> MGSSHHHHHHSQDPMLNSFKLSLQYILPKLWLTRLAGWGASKRAGWLTKLVIDLF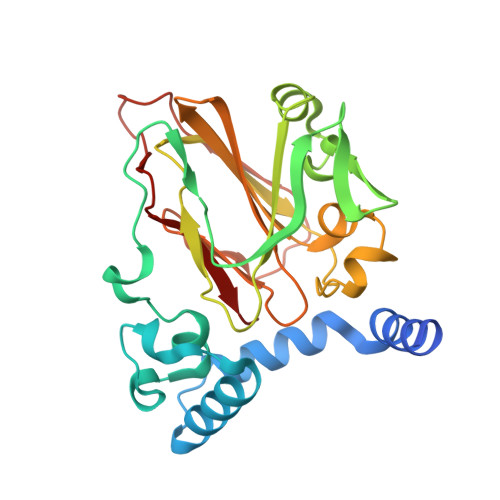VKYYKVDMKEAQKPDTASYRTFNEFFVRPLRDEVRPIDTDPNVLVMPADGVISQLGKIEEDKILQAKGHNYSLEALLAGNYLMADLFRNGTFVTTYLSPRDYHRVHMPCNGILREMIYVPGDLFSVNHLTAQNVPNLFARNERVICLFDTEFGPMAQILVGATIVGSIETVWAGTITPPREGIIKRWTWPAGENDGSVALLKGQEMGRFKLG>[2x]GYSEDRCSWRGSG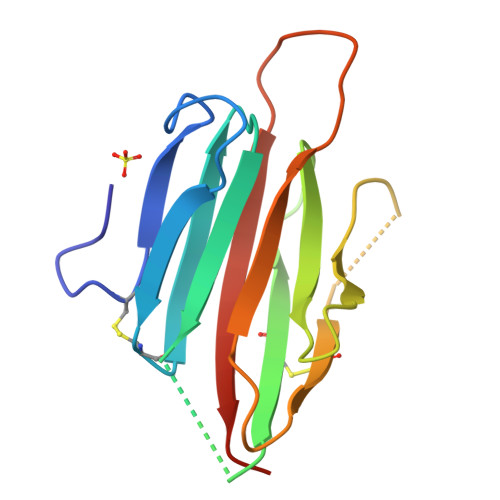LTQEPGSVGQLTLDCTEGAIEWLYPAGALRLTLGGPDPGTRPSIVCLRPERPFAGAQVFAERMTGNLELLLAEGPDLAGGRCMRWGPRERRALFLQATPHRDISRRVAAFRFELHEDQRAE>MLTGLNHLTLAVA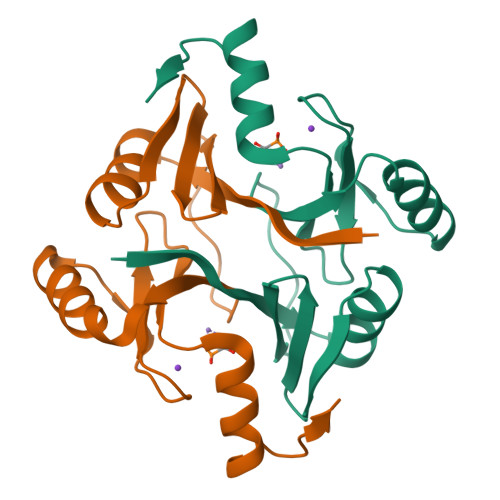DLPASIAFYRDLLGFRLEARWDQGAYLELGSLWLCLSREPQYGGPAADYTHYAFGIAAADFARFAAQLRAHGVREWKQNRSEGDSFYFLDPDGHRLEAHVGDLRSRLAACRQAPYAGMRFAD[2x]> GKDGSTAVPSLVALEKINVADIINGAQEKCVLPPMDGYPHCEGKIKWMKDMWRSDPCYADYGVDGSTCSFFIYLSEVENWCPHLPWRAKNPYEEADHNSLAEIRTDFNILYSMMKKHEEFRWMRLRIRRMADAWIQAIKSLAEKQNLEKRKRKKVLVHLGLLTKESGFKIAETAFSGGPLGELVQWSDLITSLYLLGHDIRISASLAELKEIMKKVVGNRSGCPTVGDRIVELIYIDIVGLAQFKKTLGPSWVHYQCMLRVLDSFGTEPEFNHANYAQSKGHKTPWGKWNLNPQQFYTMFPHTPDNSFLGFVVEQHLNSSDIHHINEIKRQNQSLVYGKVDSFWKNKKIYLDIIHTYMEVHATVYGSSTKNIPSYVKNHGILSGRDLQFLLRETKLFVGLGFPYEGPAPLEAIANGCAFLNPKFNPPKSSKNTDFFIGKPTLRELT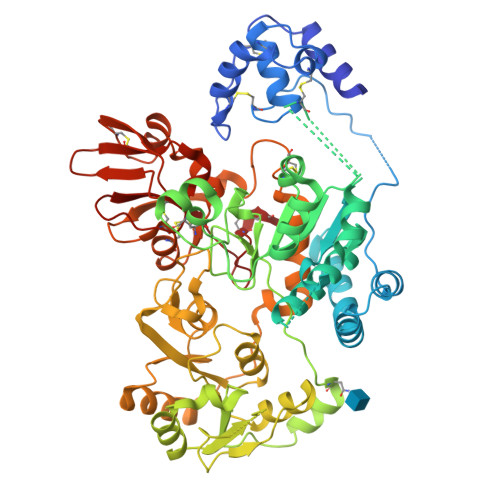SQHPYAEVFIGRPHVWTVDLNNQEEVEDAVKAILNQKIEPYMPYEFTCEGMLQRINAFIEKQDFCHGQVMWPPLSALQVKLAEPGQSCKQVCQESQLICEPSFFQHLNKDKDMLKYKVTCQSSELAKDILVPSFDPKNKHCVFQGDLLLFSCAGAHPRHQRVCPCRDFIKGQVALCKDCL N~3~-{(1S,2R)-1-benzyl-2-hydroxy-3-[(3-methoxybenzyl)amino]propyl}-N~1~,N~1~-dibutyl-1H-indole-1,3-dicarboxamide | 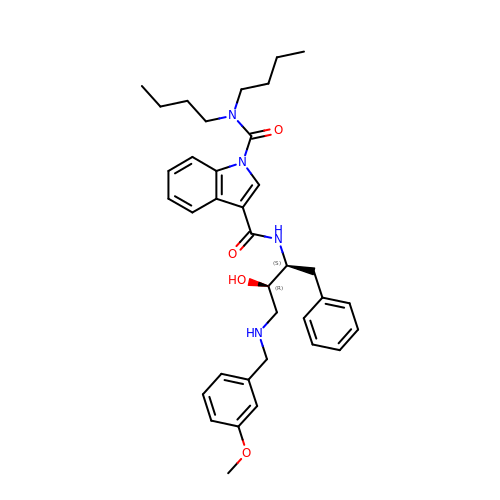C36 H46 N4 O4 | JPMPCSZOVMUPRZ-UZNNEEJFSA-N>MKVAENQKVYDITIIGGGPTGLFTAFYGGMRQASVKIIESLPQLGGQLSALYPEKYIYDVAGFPKVRAQELVDNLKEQMKKFDPTVCLEEAVDTLEKQADGIFKLVTNKQTHYSKSVIITAGNGAFQPRRLELEGTAKYEKKNLHYFVDDMNKFAGKRVVVFGGGDSAVDWTMMLEPIAEKVTIVHRRDKFRAHEHSVENLMNSRAEVSTPYVPVELIGDDKIEQVVLQHVKTEEKVIIDVDDVIVNYGFVSSLGPIKNWGLDIQKNSILVNSKMETNIPGIYAAGDICTYEGKVKLIACGFGEAPTAVNNAKAYFDPNAKLQPMVSSSMF[4x]

Bacillus cereus (Bc) encodes three FNR paralogs, two of which have assigned distinct biological functions in bacillithiol disulfide reduction and flavodoxin (Fld) reduction. In this study, we have assigned a function to FNR1, in which the His residue is replaced by a conserved Val, in the reduction of the heme-degrading monooxygenase IsdG, ultimately facilitating the release of iron in an important iron acquisition pathway. The Bc IsdG structure was solved, and IsdG-FNR1 interactions were proposed through protein–protein docking. Mutational studies and bioinformatics analyses confirmed the importance of the conserved FAD-stacking residues on the respective reaction rates, proposing a division of FNRs into four functionally unique sequence similarity clusters likely related to the nature of this residue.

To investigate if the interchange of Val to His in FNR1 and His to Val in FNR2 could explain the differences in the efficiencies of Fld or IsdG reduction, we generated cross-mutants of the two proteins, FNR1V329H and FNR2H326V. In the case of FNR2H326V, the replacement of His with Val resulted in a nearly 3-fold decrease in the turnover number in the reduction of NrdI and a 15-fold decrease in the reduction rate of Fld1, as compared to our previous studies on the wild-type protein. In contrast, the FNR2H326V crystal structure revealed interesting and unusual features, including an asymmetric rotation of the NAD(P)H-binding domain relative to the FAD-binding domain in the two monomers of the biological dimer. Interestingly, the second monomer has adopted a different conformation of the NAD(P)H-binding domain, resulting in an asymmetric dimer. This conformation is more closed, resembling the low-molecular-weight (low Mr) TrxR structure, where a different conformational change is required for catalysis than for FNRs. Furthermore, the second monomer with the alternative conformation completely lacks electron density corresponding to the FAD cofactor and is, in fact, an apoprotein. In the conformation seen for the FAD-free monomer, the position conventionally occupied by FAD is not stacked by the C-terminal subdomain of the opposite monomer. Moreover, the total loss of the FAD cofactor in one monomer, and a 100% occupancy in the other has never been described previously. Additionally, the asymmetry in FNR2H326V indicates that the enzyme may exhibit a negative cooperativity with respect to the binding of FAD, possibly affecting the reaction rate of Fld reduction.> ETPF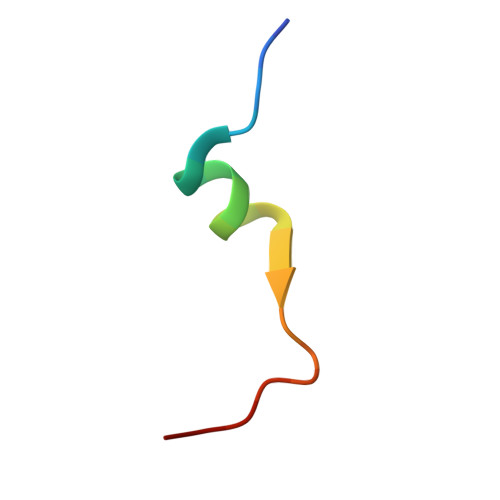TWEESNAYYWQPYALPL> MYHQEPYISKPEERFKAPPILPPHLLQVILNKDTGISCDPALLPEPNHVMLNHLYALSIKDGVM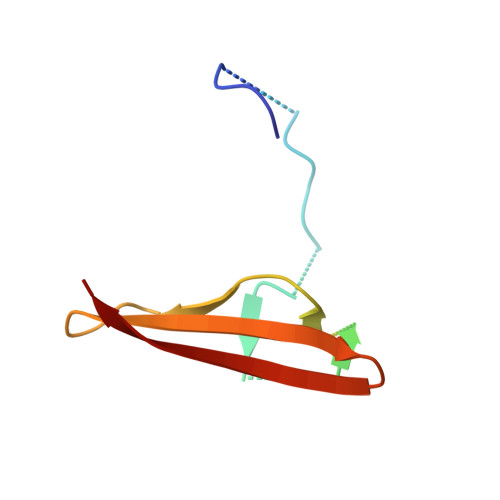VLSATHRYKKKYVTTLLYKPI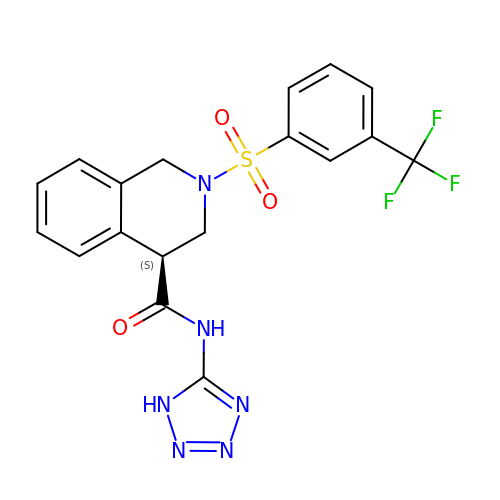(4S)-N-(1H-tetrazol-5-yl)-2-[3-(trifluoromethyl)benzene-1-sulfonyl]-1,2,3,4-tetrahydroisoquinoline-4-carboxamide | C18 H15 F3 N6 O3 S | HRYBICGLAWEIFK-OAHLLOKOSA-N> GAMALIEVEKPLYGVEVFVGETAHFEIELSEPDVHGQWKLKGQPLAASPDCEIIEDGKKHILILHNCQLGMTGEVSFQAAQ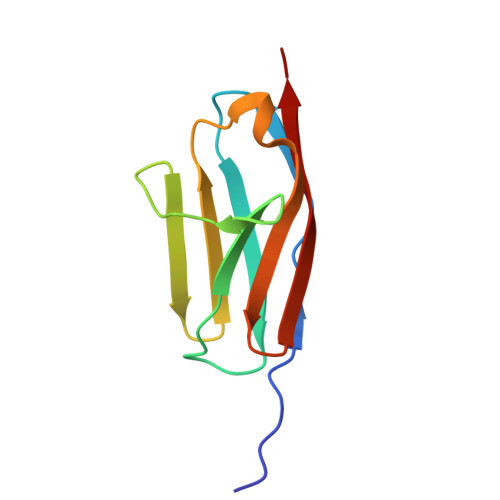TKSAANLKVKEL> SGSGSTEEEEALLRWFQTLLAKFDELVKQLGDPRLLEEARRLQERLEEAKKRGDKRTIKQLAALLQMFVLIAQIFQLVEELGDPKLLEQAKRLLERLKEAVERGDEETIKELLDLAHMTYLIAQIFQLVEQLGDPRLLELAKELLKRLKEAQERGDRRTIERLLRLVQMTYLIAQIFQLVRQLGDPR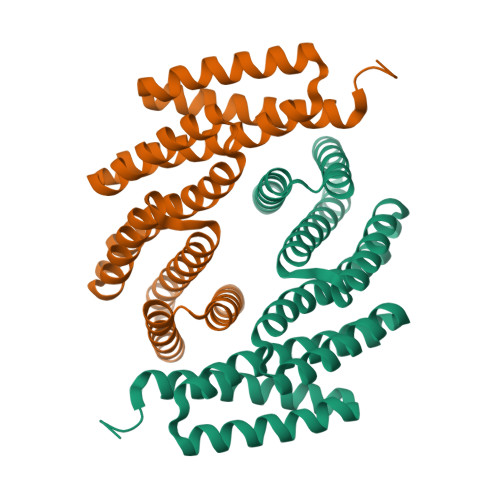LLETAKTLLTLLKLAFEEGDELLIKSLLTLVAETYRQAAAEQ>MPKPYVAINMAELK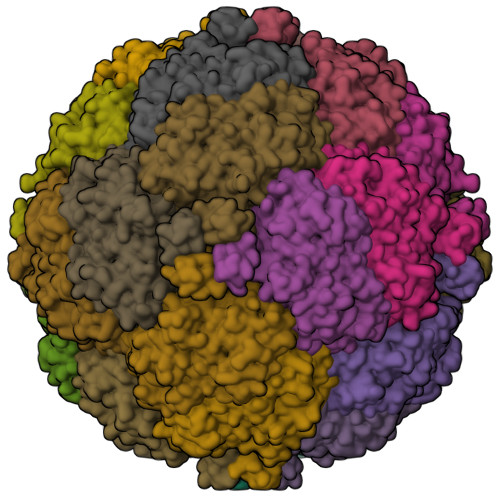NEPKTFEMFASVGPKVCMVTARHPGFVGFQNHIQIGILPFGNRYGGAKMDMTKESSTVRVLQYTFWKDWKDHEEMHRQNWSYLFRLCYSCASQMIWGPWEPIYEIIYANMPINTEMTDFTAVVGKKFAEGKPLDIPVISQPYGKRVVAFAEHSVIPGKEKQFEDAIVRTLEMLKKAPGFLGAMVLKEIGVSGIGSMQFGAKGFHQVLENPGSLEPDPNNVMYSVPEAKNTPQQYIVHVEWANTDALMFGMGRVLLYPELRQVHDEVLDTLVYGPYIRILNPMMEGTFWREYLNEQAWRHPQFGG[6x]>[3x]MHHHHHHQQEALGMVET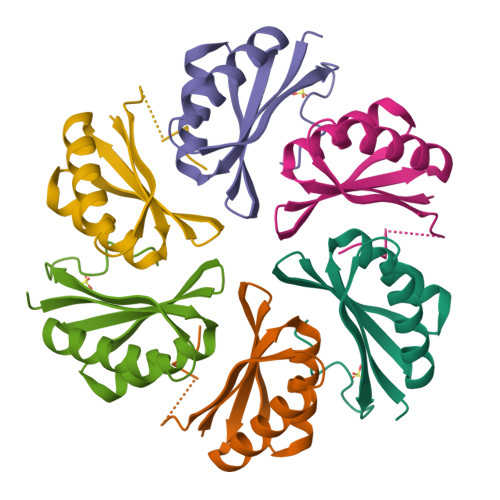KGLTAAIEAADAMVASANVMLVGYEKIGLGLVTVIVRGDVGAVKAATDAGAAAARNVGEVKAVHVIPRPHTDVEKILPKGISQ>MVMKQTKQTNILAGAAVIKVLEAWGVDHLYGIPGGSINSIMDALSAERDRIHYIQVRHEEVGAMAAAADAKLTGKIGVCFGSAGPGGTHLMNGLYDAREDHVPVLALIGQFGTTGMNMDTFQEMNENPIYADVADYNVTAVNAATLPHVIDEAIRRAYAHQGVAVVQIPVDLPWQQIPAEDWYASANSYQTPLLPEPDVQAVTRLTQTLLAAERPLIYYGIGARKAGKELEQLSKTLKIPLMSTYPAKGIVADRYPAYLGSANRVAQKPANEALAQADVVLFVGNNYPFAEVSKAFKNTRYFLQIDIDPAKLGKRHKTDIAVLADAQKTLAAILAQVSERESTPWWQANLANVKNWRAYLASLEDKQEGPLQAYQVLRAVNKIAEPDAIYSIDVGDINLNANRHLKLTPSNRHITSNLFATMGVGIPGAIAAKLNYPERQVFNLAGDGGASMTMQDLATQVQYHLPVINVVFTNCQYGFIKDEQEDTNQNDFIGVEFNDIDFSKIADGVHMQAFRVNKIEQLPDVFEQAKAIAQHEPVLIDAVITGDRPLPAEKLRLDSAMSSAADIEAFKQ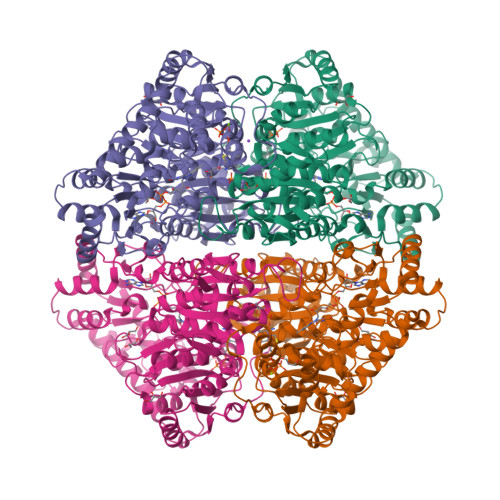RYEAQDLQPLSTYLKQFGLDDLQHQIGQGGF[2x]6-chloropyrazine-2-carboxylic 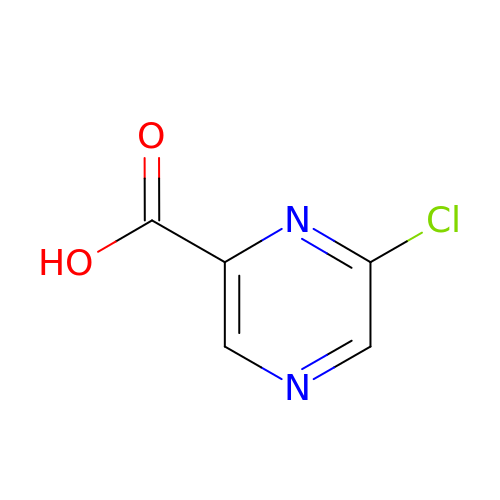acid | C5 H3 Cl N2 O2 | KGGYMBKTQCLOTE-UHFFFAOYSA-N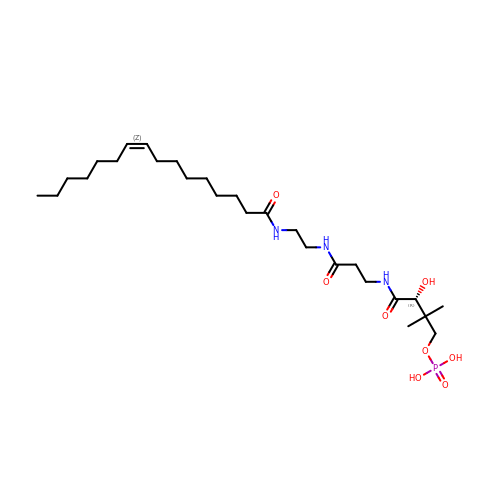N~3~-{(2R)-4-[(dihydroxyphosphanyl)oxy]-2-hydroxy-3,3-dimethylbutanoyl}-N-(2-{[(9Z)-hexadec-9-enoyl]amino}ethyl)-beta-alaninamide | C27 H52 N3 O8 P | GXMQTIIOLQTNTK-JRUKXMRZSA-N We apply the force distribution analysis to I27, an IG domain of the muscle protein titin and one of the most robust protein domains known. We have determined the first high-resolution crystal structure of I27, a cornerstone for the interpretation of force spectroscopy experiments and crucial for our analysis. We present here the first force distribution network in a protein at atomic detail, thereby revealing the force-bearing scaffold rendering I27 mechanically robust. The A'G strand, known to be crucial for mechanical resistance, forms a mechanical clamp.

There are six I27 molecules in the asymmetric unit arranged around the local non-crystallographic 6-fold axis, with the N-termini of I27 closest to the local axis and the C-termini pointing outward. The entire amino acid sequence from residue 1–89 is visible in electron density (except L89 in chain E), as well as an additional 3–4 residues left from the TEV cleavage site after the N-terminal H6-tag (-AMA- in chain A; none in chain B; and -GAMA- in chains C–F, see Methods). As a comparison, the RMSD between non-crystallographic symmetry-related chains in the I27 crystal structure ranges from 0.16–0.35Å. The present crystal structure of I27 represents an improved model for further studies because it does not contain potential structural perturbations introduced by unwanted mutations, and due to the high quality diffraction data, with overall coordinate error of 0.15Å. Overall, there are more and shorter H-bonds in the crystal structure comparing to the previously described NMR structure. An additional H-bond between E3 and S26 and a stronger bond between K6 and E24 are found between strands A and B. While the hydrogen bonding between the A' and G strand largely overlaps, the interaction between Y9-N83 is absent but E12-K87 are within interaction distance, the latter supposedly adding resistance. Of the two residues mutated in the NMR structure, T78 (first residue of strand G) makes a side chain H-bond interaction with the carbonyl oxygen of L2 (preceding strand A) which is absent in the NMR structure and which could potentially add further mechanical resistance to I27. A number of structural features, such as the A'G interstrand hydrogen bonds or the interactions involving T78, which was absent in the NMR structure due to the T78A mutation, are part of the force-bearing network. The determination of a refined crystal structure thus served as an important basis for our force distribution analysis.

>GAMALIEVEKPLYGVEVFVGETAHFEIELSEPDVHGQWKLKGQPLAASPDCEIIEDGKKHILILHNCQLGMTGEVSFQAANTKSAANLKVKEL[4x];> GAMALIEVEKPLYGVEVFVGETAHFEIELSEPDVHGQWKLKGQPLAASPDCEIIEEGKKHILILHNCQLGMTGEVSFQAANTKSAANLKVKEL;> GAMALIEVEKPLYGVEVFVGETAHFEIELSEPDVHGQWKLKGQPLAASPDCEIIEDGKKHILILHNCQLGMTGEVSFQAAQTKSAANLKVKEL> MGG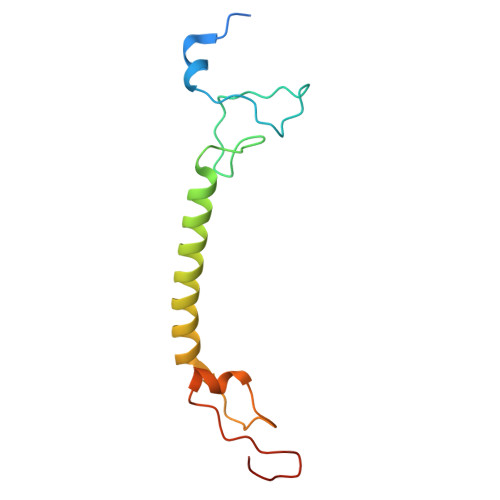HDHHHPSVPEPPYAKYLANKSHYCPPDFHYSREIYAPYGGYFNDPKGWRTNTAIATLVMLAGAYAVFCFGNAREERLRAPKGWIPSQLWNDNVPTPVDYRGKVLKDE> PHMKYYGNGVTCGKHSCSVDWGKATTCIINNGAMAWATGGHQGN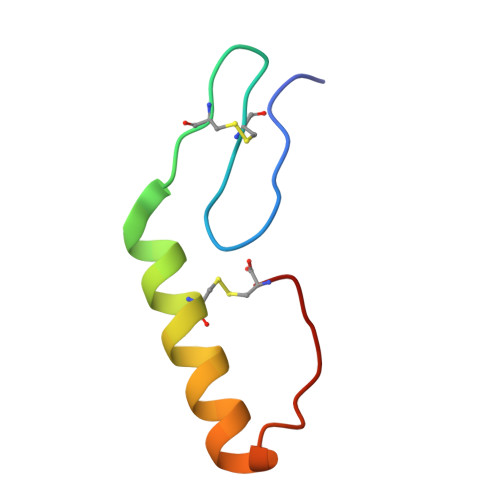HKC The bacterial member PspA is part of the phage shock protein (psp) response that maintains structural integrity of membranes under stress conditions such as temperature and infection. The main effector of the Psp system is PspA, a 25 kDa protein consisting of six α-helices connected by short loops and an elongated hairpin, where the N-terminal helix α0 of the protein remains unfolded in the absence of membranes. Interestingly, PspA is related to eukaryotic and archaeal endosomal sorting complexes required for transport (ESCRT)-III proteins and has a similar structure. Here, we show that rods of bacterial ESCRT-III protein PspA internalize and thin membrane tubules by overcoming the required bending energy through progressive membrane binding of the N-terminal helix in the PspA assembly.

Due to the critical role of helix α0 in membrane interaction, we also prepared and refolded an N-terminally truncated PspA including helices α1-5 in the presence of EPL liposomes. For the truncated PspA α1-5 sample, the total diameter distribution was narrower and ranged from 235 to 290 Å, with two maxima at 255 Å and 275 Å that were closer but not identical to the apo distribution of WT PspA. In the PspA α1-5 + EPL sample, we determined a total of five cryo-EM structures with resolutions ranging from 3.8 to 5.4 Å supported by visible side-chain details. For the α1-5 PspA variant, we found only five rod diameters (235, 250, 270, 280, and 290 Å), whereas two different symmetries (C1 and C2) could be identified for the diameter of 270 Å. None of these structures contained any additional lipid density in the rod lumen. Although the PspA mutant lacking helix α0 shows no structural alterations in the helical rod structure, it can no longer tubulate EPL membranes. In support of this analysis, when we abolished the α0–membrane interaction by removing helix α0 lacking this binding energy contribution, we did not observe any membrane internalization in the lumen of the PspA (α1-α5) rods in the cryo-EM images. Interestingly, when the protein was reconstituted in the presence of membranes, the ATPase activity was increased by ~210%, while the activity of PspA α1-5 was not affected in the presence of membranes.

>MGSSHHHHHHSSSAALEVLFQGPAPEDLLERLLGEMELELIELRRALAQTIATFKSTERQRDAQQLIAQRWYEKAQAALDRGNEQLAREALGQRQSYQSHTEALGKSLGEQRALVEQVRGQLQKLERKYLELKSQKNLYLARLKSAIAAQKIEEIAGNLDNASASSLFERIETKILELEAERELLNPPPSPLDKKFEQWEEQQAVEATLAAMKARRSLPPPSS[60x]> GAMGKLCENQQEIYAAYRVANLLGVYEDCSPNGFYQRWKQKNAFMKAQAEEFGIGSTDHFIDDVERIVDQRRAETEWKNADAWKNGTAAFGARYLTPEMYLDYELKSIQLAFATYKGELVGNHKCHVYTEDEKRAFYDANQDLFTRYHGDLFSYEEVDLIIEKWLKVQEYQDIIESVVANTHLNETTVNEISAQDVSDEKSDNAVRWITEFEKIWNQMQEEKRLREDKSCPEETKSESSIGNCGHCYYVSSIHGDDANDGTEDQPLKSLYAVNRLDLQPGDQVLLERGSVFENQFLHLNVQGTKEQPIYIGAYGNGAKPLIQTNGQGIWYQDYGNELDAPTHVYRGYVSSAVLLYDCEYLTVENLEISNKGGVFGETYSAPHKMNRTGVAGIAKNRGTLHEIHLSNLYIHDVEGNVYDKHMNNGGIYFTCLKPEAEEKTGVARYENVSVRGCHLKRTSRWGIAVGYSYKCKEFMTAELPDELFERYGHHNIYIADNYVEEIGGDGITVMYAMKPLVEYNSGDSCALEMNDRYYTEPEDRAGKVAAGIWPWKCKDALLTYNEMRDMRLNQDSMAWDADSGDGTLYQYNYSHLNEGGCVMFCLEEAIHNEFRYNVSVDDLGGLISPSGNPDAWIHHNVFYRRAEVPFVRPHMDDGKYVAEENEIHLI

E. ramulus and R. hominis also shared similar growth profiles on LNT, which was consistent with the presence of a functional GH136. The N-terminal (ErLnb136I) and the C-terminal (ErLnb136II) regions of the E. ramulus GH136 share homology to RhLnb136I and RhLnb136II, respectively, suggestive of the fusion of ErLnb136I and ErLnb136II to form an active enzyme (ErLnb136). This is supported by the identical specificity and similar catalytic efficiencies of ErLnb136 and RhLnb136. Moreover, intimate interaction of the two ErLnb136 domains is consistent with the cooperative unfolding profile of the enzyme. These data justified the use ErLnb136 to study the architecture of the two subunits/domains compulsory for activity within GH136.

The crystal structures of selenomethionine (SeMet)-labelled and native ErLnb136 were determined at 1.4 and 2.0 Å resolution, respectively. The C-terminal catalytic domain (ErLnb136II, from AA 242-663) assumes a β helix fold similar to the bifidobacterial homolog LnbX. The LNB molecule bound in the active site is recognized by ten potential hydrogen bonds and aromatic stacking of the Gal unit onto W548. Interestingly, the GlcNAc sugar ring of LNB in ErLnb136 adopts an 4E conformation (φ = 232° and ψ = 68°) with the O1-OH in a pseudo-axial position to form a direct hydrogen bond with the acid/base catalyst (D568). Moreover, the D575 Oδ2 of the nucleophile is positioned appropriately for nucleophilic attack on the anomeric carbon of the GlcNAc at 3.2 Å. The N-terminal domain (ErLnb136I, from AA 7-224) consists of 8 α-helices (α1-α8) and assumes a previously unknown fold, stabilized by the central helix α1. The ErLnb136I domain embraces the sides and back of the β helix domain. These extensive inter-domain interactions (solvent inaccessible interface ≈1618 Å2), stabilize the protein structure with ΔG = −17 kcal mol−1. Remarkably, the α6-α7 loop of ErLnb136I forms a part of the active site with the solvent accessible sidechain of Y145 positioned near the active site (5.7 Å to the GlcNAc O1 atom of LNB). The Y145A mutant showed a 4.9-fold higher KM, suggesting that this residue contributes to substrate interactions, possibly at the +1 subsite.>[2x]MSLDVDSKTLIHAGKLIDGKSDQVQSRISIVIDGNIISDIKKG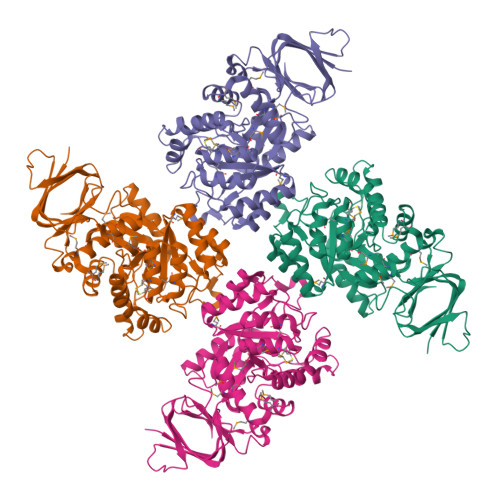FISSNDFEDYIDLRDHTVLPGLMDMHVHFGQEYQSKAQAPIKVEREMQAILATQHAYVTFKSGFTTVRQVGDSGLVAISLRDAINSGKLAGPRIFAAGKTIATTGGHADPTNGKAVDDYDYPVPEQGVVNGPYEVYAAVRQRYKDGADGIKITVTGGVLSVAKSGQNPQFTQEEVDAVVSAAKDYGMWVAVHAHGAEGMKRAIKAGVDSIEHGTFMDLEAMDLMIENGTYYVPTISAGEFVAEKSKIDNFFPEIVRPKAASVGPQISDTFRKAYEKGVKIAFGTDAGVQKHGTNWKEFVYMVENGMPAMKAIQSATMETAKLLRIEDKLGSIESGKLADLIAVKGNPIEDISVLENVDVVIKDGLLYEGHHHHHH Here we dissected the structural basis for neuropeptide-gated activity of a neuropeptide-gated DEG/ENaC, FMRFamide-gated sodium channel 1 (FaNaC1) from the annelid worm Malacoceros fuliginosus, using cryo-electron microscopy. We solved high-resolution structures of FaNaC1 alone, with full agonist FMRFa, with partial agonist ASSFVRIa, and with both FMRFa and pore-blocker diminazene, identifying the ligand-binding site and elucidating the conformational changes induced by ligand binding. Each subunit comprises a minimal N terminus and a nonresolved 63-amino acid C terminus facing the intracellular side, two transmembrane segments (TM1 and TM2), and a large extracellular domain. The FaNaC1 structures presented here capture a ligand-free resting state, two ligand-bound desensitized states and a ligand-bound dilated channel state.

Preparations of FaNaC1 alone and with FMRFa (30 μM) yielded 3D reconstructions with a global resolution of 2.7 and 2.5 Å, respectively. In the FaNaC1/FMRFa structure, we observed a discrete cryo-EM density in a small pocket at the upper corner of each subunit, which fits a single FMRFa molecule. The FMRFa-binding pocket is formed by α-helical segments α1–α3a (residues V87 to F144), the β6–β7 loop of the same subunit (residues D234 to G241), and partly by α6 from the adjacent subunit (G423–K428). The basis for ligand recognition appears to be mostly hydrophobic interactions. The FMRFa N-terminal phenylalanine residue (F1) is positioned near the entrance to the pocket and the M2 side chain orients downward between α2-F129, β6–β7 loop-I236 and M238, and α6-F431. FMRFa R3 orients upward: the density for the guanidino moiety in our map is relatively weak, but the modeled side chain is 4–6 Å from polar side chains α1-D101 and β6–β7 loop-E235 and R237. Finally, FMRFa F4 and C-terminal amide sit deep in the pocket, with the F4 side chain surrounded as closely as 3.5–4.6 Å by the hydrophobic side chains of α1-F97, P103, α2-V122, A126 and F129, and β6–β7 loop-P240. Additionally, FMRFa M2 main chain carbonyl oxygens are 2.5–3.1 Å from the FaNaC1 α2-Q133 amide side chain, indicative of a potential polar interaction. In both ligand-bound structures, however, the channel pore appears closed, with radii of ~1 Å at the level of G503 and G506 in TM2a (G3′ and G6′ in a TM2 numbering scheme). Thus, FMRFa- and ASSFVRIa-bound channels have probably adopted a desensitized state in the prolonged presence of agonist, in accord with the large decrease in current amplitude that occurs within ~2 s of FMRFa application, especially at higher FMRFa concentrations (for example).

>[3x]MSAIRDVMTKFAEQTTMHGVPKVINAKSSMGRLFWSLVCLAAGAMFCLQMSEVLQRYFSYPKKVTVEVVPTPVPFPSISICNMRNLDVHILNTLNRMFIEDDRPFSNINKSEHEFIRAYMKKVAKYAPLFWNYQDEYPEVFQEIFSRTTFSANIDPEVIALAAVQLEGFVVNCHYAGHRCNKTRDFYRFFDPYYFNCFTYKAHEPTDIEDNLSEGIENGWSSILLSGSGMLDKNDEIRMLPGLHEWRSAVSASEGVRVVIHPPSTTPYPFTEGYDVPPGFSASFGIHPRRNIRIGPPHGNCSDKNPFGDGTERYRLMACQKMCMQHYIVETCGCADVGLPKLPLQANISWCRDDDNFPDECMFTASEECLQLLMQLHNRIKCARSIKSKITKNTTAMEACNCFPPCDEVSYDVSYSLSKWPSAGYEGDAAYFDVFGIEKFNERFNKTGTQGKYELFTKYFNVSNREESMKDFARLNVYIADSNVVKTQESEDYTRNQLVSDIGGQLGLWVGISLITLAEVLELIIDLFRLFSKHTYRSVPVIRQSIKYKDKRNGAEMNYDTRYSQSNGGPHARYLHHGHSIPKHPPELPDTSLALEVLFQ;>FMRFX[3x]>MDNDDKKPDALIHLRVPAEVKGRWVKESRLEGMKLTDWITGRVEAKALSIAEVLEEAAAMARSLEDSPIFYRNKLCADGIVTIQQQAARFSAATDDATRLDAALWAREGYQLLSSGLPDSYSGAVPNEGRTG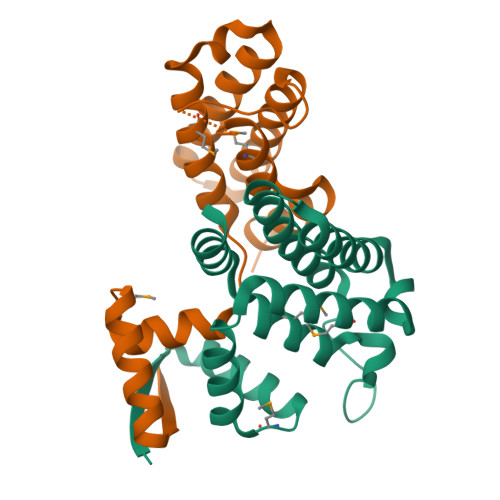WVTASQMARLFGGEALWIERCQQELGGAGKEDGR[2x]> MGKLPESPKRAEEIWQQSVIGDYLARFKNDRVKALK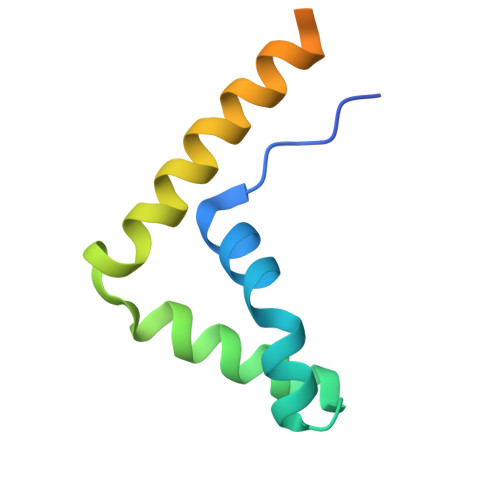AMEMTWNNMEKKEKLMWIKKAAEDQKRYERELSEMRAPPAATNSSKKLEHHHHHH3-[(4-AMINO-2-METHYLPYRIMIDIN-5-YL)METHYL]-2-(1-CARBOXY-1-HYDROXYETHYL)-5-(2-{[HYDROXY(PHOSPHONOOXY)PHOSPHORYL]OXY}ETHYL)-4-METHYL-1,3-THIAZOL-3-IUM 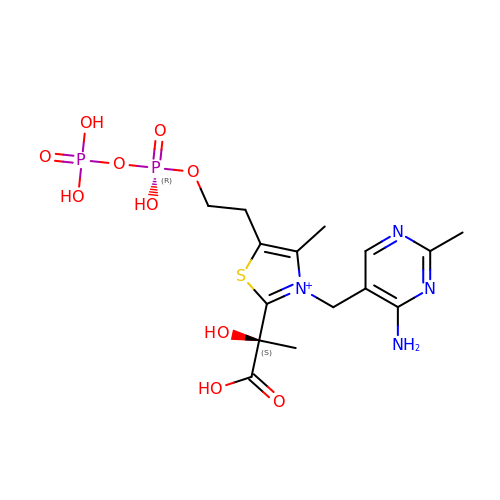| C15 H23 N4 O10 P2 S | TVDSMGSBVYONNB-OAHLLOKOSA-O(2R)-2-{[(2R)-2-{[(2S)-2-{[(2R)-2-hydroxypropyl]oxy}propyl]oxy}propyl]oxy}propan-1-ol 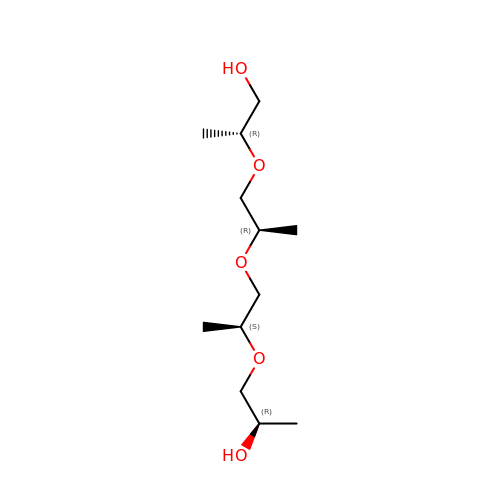| C12 H26 O5 | QVHMSMOUDQXMRS-WISYIIOYSA-N> GAMGSMVKLAEFSRTATFAWSHDKIPLLVSGTVSGTVDANFSTDSSLELWSLLAADSEKPIASLQVDSKFNDLDWSHNNKIIAGALDNGSLELYSTNEANNAINSMARFSNHSSSVKTVKFNAKQDNVLASGGNNGEIFIWDMNKCTESPSNYTPLTPGQSMSSVDEVISLAWNQSLAHVFASAGSSNFASIWDLKAKKEVIHLSYTSPNSG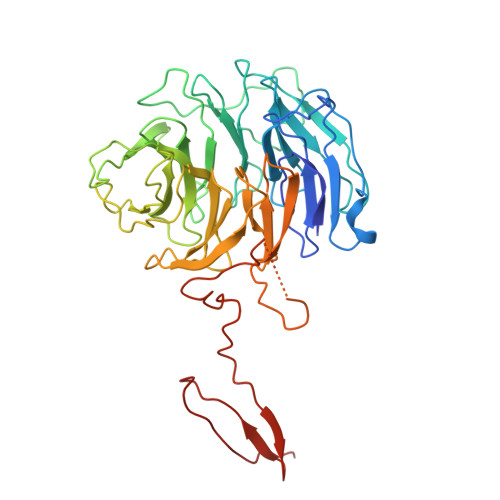IKQQLSVVEWHPKNSTRVATATGSDNDPSILIWDLRNANTPLQTLNQGHQKGILSLDWCHQDEHLLLSSGRDNTVLLWNPESAEQLSQFPARGNWCFKTKFAPEAPDLFACASFDNKIEVQTLQNLTNTLDEQETETKQQESETDFWNNVSREESKEKPSVFHLQAPTWYGEPSPAAHWAFGGKLVQITPDGKGVSITNPKISG>AEGVGNSSGDWHCDTKWMGDHVITKSTRTWVLPTYGNHLYGPINFDGTTGSGANAAYAGYKTPWGYFDFNRFHCHFSPRDWQRLINNHTGIRPKGLKIKVFNVQVKEVTTQDSTKTIANNLTSTVQIFADENYDLPYVLGSATQGTFPPFPNDVFMLPQYAYCTLQGNSGKFVDRSAFYCLEYFPSQMLRTGNNFEFQFKFEEVPFHSGWAQSQSLDRLMNPLLDQYLIGDYGTDASGNLIYHRAGPNDLNEFYKNWAPAPYECIQNINSSDNTKNANSINGSNSTNKWGLQGRQAWDAPGFVQASTYEGAAAGQSLLNGVLTFDKSSATTSSPAATAVNRTIEDEIQGTNNFGNARNNIV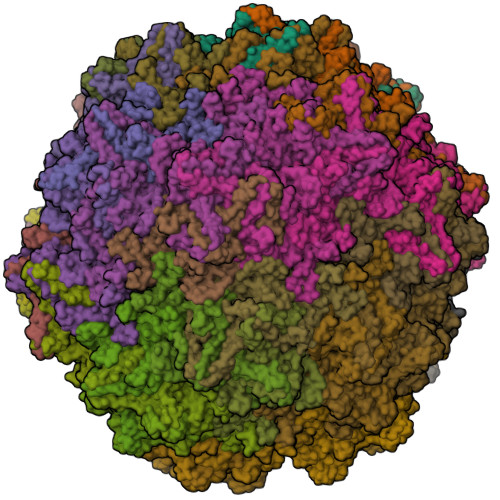AINQQTKGTNPTTGSTSQFETMPGMVWSNRDIYLQGPIWAKIPNTDGHFHPSPRMGGFGLKHPPPMILIKNTPVPADPPTTFNPMPQTSFITEYSTGQVTVEMLWEVQKESSKRWNPEVQFTSNFGTSDPAVDGIPFGINNLGTYVESRPIGTRYISKHL[60x]>MLETYDWNNKLTYLKNTRDLYYNDDYVSFLVNTVWKITKPVHIVDYGCGYGYLGLVLMPLLPEGSKYTGIDSGETLLAEARELFRLLPYDSEFLEGDATEIELNDKYDIAICHAFLLHMTTPETMLQKMIHSVKKGGKIICFEPHWISNMASYLLDGEKQSEFIQLGVLQKLFESDTQRNGKDGNIGMKIPIYLSELGVKNIECRVSDKVNFLDSNMHHNDKNDLYQSLKEEGIAGDPGDKQQFV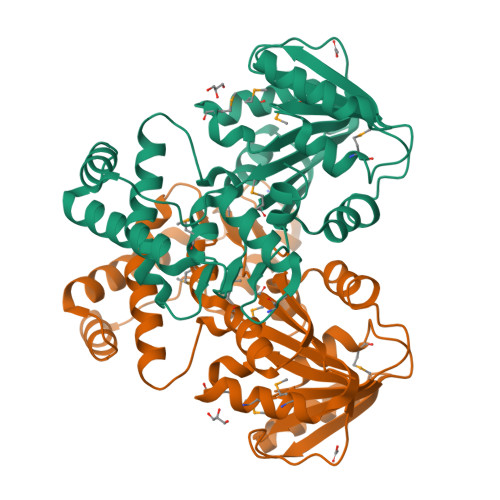ERLIARGLTYDNALAQYEAELRFFKALHLHSSLVYAPNMKITFGEIECLEHHHHHH[2x]>[8x]MKYILVTGGVISGVGKGVIASSFGTLLKSCGLDVTSIKIDPYINIDAGTFSPYEHGEVYVLDDGAEVDLDLGNYERFLDVTLHRDNNITTGKIYKLVIEKERTGEYLGKTVQVVPHITDAIQEWVERVAQTPVQGSSKPQVCIVELGGTIGDIEGMPFVEAFRQFQFRVKRENFCLAHVSLVPLPKATGEPKTKPTQSSVRELRGCGLSPDLIVCRSEKPIGLEVKEKISNFCHVGPDQVICIHDLNSIYHVPLLMEQNGVIEYLNERLQLNIDMSKRTKCLQQWRDLARRTETVRREVCIAVVGKYTKFTDSYASVVKALQHAALAVNRKLELVFIESCLLEEETLHSEPSKYHKEWQKLCDSHGILVPGGFGSRGMEGKIRACQWARENQKPLLGICLGLQAAVIEFARNKLGLKDANTTEIDPNTANALVIDMPEHHTGQLGGTMRLGKRITVFSDGPSVIRQLYGNPKSVQERHRHRYEVNPKY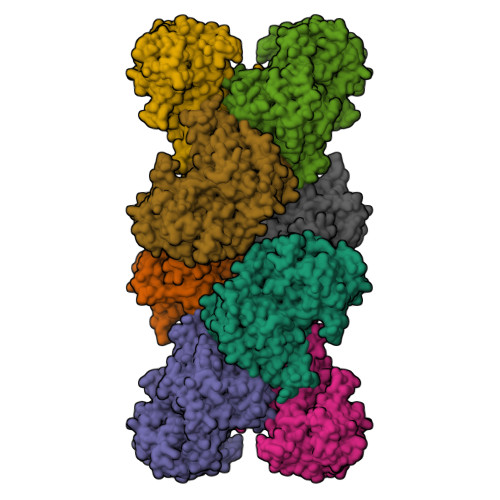VHLLEEQGMRFVGTDVDKTRMEIIELSGHPYFVATQYHPEYLSRPLKPSPPFLGLILASVDRLNQYIQRGCRLS>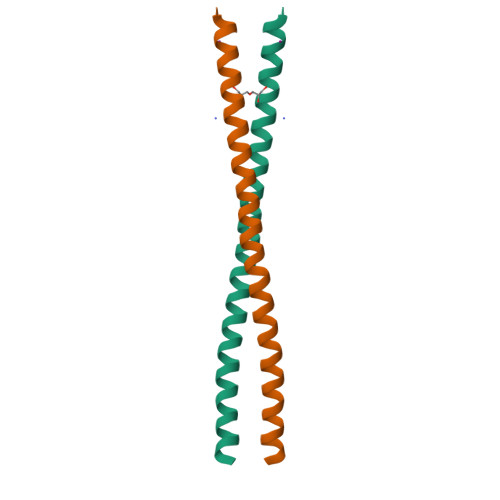 KLKLVGMEKEQREQEEKQRKAEELLQELRHLKIKVEELENERNQYEWKLKATKAEVAQLQEQVALKDAEIERLHSQLSRTA> SMRGPPAWAGDEAWRRGPAAPPGDKGRLRPAAAGLPEARKLLGLAYPERRRLAAAVGFLTMSSVISMSAPFFLGKIIDVIYTNPTVDYSDNLTRLCLGLSAVFLCGAAANAIRVYL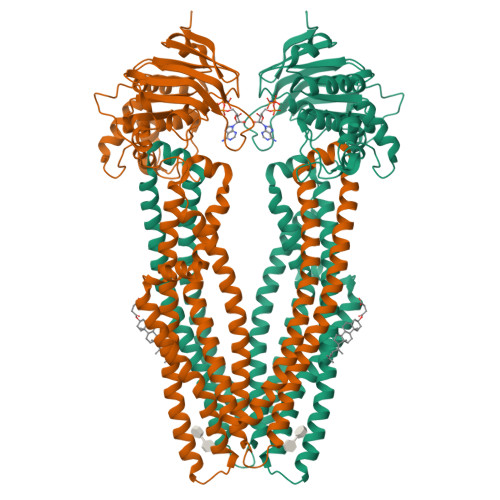MQTSGQRIVNRLRTSLFSSILRQEVAFFDKTRTGELINRLSSDTALLGRSVTENLSDGLRAGAQASVGISMMFFVSPNLATFVLSVVPPVSIIAVIYGRYLRKLTKVTQDSLAQATQLAEERIGNVRTVRAFGKEMTEIEKYASKVDHVMQLARKEAFARAGFFGATGLSGNLIVLSVLYKGGLLMGSAHMTVGELSSFLMYAFWVGISIGGLSSFYSELMKGLGAGGRLWELLEREPKLPFNEGVILNEKSFQGALEFKNVHFAYPARPEVPIFQDFSLSIPSGSVTALVGPSGSGKSTVLSLLLRLYDPASGTISLDGHDIRQLNPVWLRSKIGTVSQEPILFSCSIAENIAYGADDPSSVTAEEIQRVAEVANAVAFIRNFPQGFNTVVGEKGVLLSGGQKQRIAIARALLKNPKILLLDEATSALDAENEYLVQEALDRLMDGRTVLVIAHHLSTIKNANMVAVLDQGKITEYGKHEELLSKPNGIYRKLMNKQSFISA>MSDKIIHLTDDSFDTDVLKADGAILVDFWAEWCGPCKMIAPILDEIADEYQGKLTVAKLNIDQNPGTAPKYGIRGIPTLLLFKNGEVAATKVGALSKGQLKGFLDANLA[2x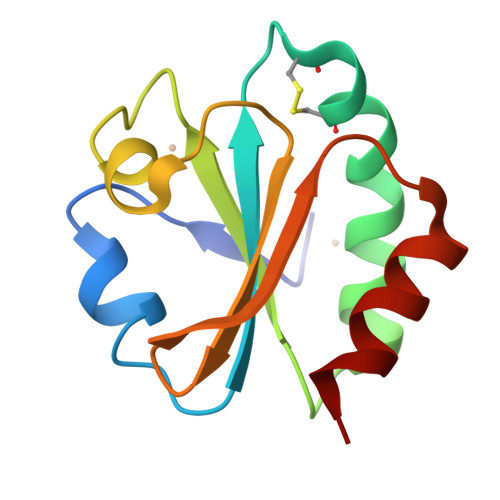]>[2x]MSLNRLLSAARRSDRRASALSSFRSLSASPALAPSAASPPAPPPPTAMIYDRAAEAIKSKLRQLENPDPRFLKHGNPRPALSDHTRILAAPETRVTTLPNGLRVATESSLAARTATVGVWIDAGSRFETEETNGTAHFLEHMIFKGTERRNARELEEEIENMGGHLNAYTSREQTTYYAKVTDSDVPQALDILADILQNSRFEENRISRERDVILREMEEVEGQTEEVIFDHLHATAFQYTPLGRTILGPAQNIKTITKAHLQSYIQTHYTAPRMVIAASGAVKHEDIVEQVKKLFTKLSTDATTTAQLVAKEPAIFTGSEVRMLDDDIPLAQFAVAFEGASWKDPDSIALMVMQAMLGSWNKTAGGGKHMGSELAQRVGINEVAESIMAFNTNYKDTGLFGVYAVAKPDCLDDLSYAIMQETTKLVYRVSEDDVTRACNQLKSSLLLHIDGTSPVAEDIGRQLLTYGRRIPFAELFARIDAVDASTIKRVANRFIYDKDVAIAAMGPIQRLPDYNWFRRRTYWNRY;>[2x]MYRAAASSFRRHLKGHGSKLGSTRSSTSAAVAARTSKGGLFSWLTGERSSSLPSLDIPLGGVVLPDPLPDSVEQSKTKITTLSNGLKIASETSPNPAASIGLYLDCGSIYETPFSSGASHLLERMAFKSTTNRSHFRIVREVEAIGGNIGASASREQMGYTFDALKTYVPQMVELLVDCVRNPAFLDWEVNEELRKVKAELGELSNNPQGLLLEAIHSAGYSGALAYPLLAPEAALNRLDGPSLE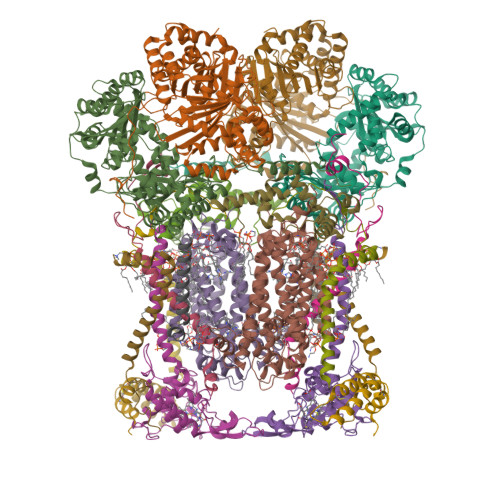EFVAENYTAPRMVLAAAGVEHEELVSIAEPLLSDLPNVPRPDEPKSVYVGGDFRRHGESGGTHVALAFEVPGGWHKEKDAIVLTVLQMLMGGGGSFSAGGPGKGMHSRLYLRVLNEYQQIQSFSAFNSIFNNTGLFGIYASTSPDFAPKAVDIAAKELIAIASPGQVTQVQLDRAKKSTKSAVLMNLESRMIASEDIGRQILTYGERKPLEQFLKAVDEITLNDITKISQKIISSPLTMASYGDVLSVPSYESVNRKFHAK;>MTIRNQRFSLLKEPISSTLNQHLIDYPTPSNLSYWWGFGSLAGICLVIQIVTGVFLAMHYTPHVDLAFNSVEHVMRDVEGGWLLRYMHANGASMFFIVVYLHIFRGLYYASYSSPREFVWCLGVVIFLLMIVTAFTGYVLPWGQMSFWGATVITSLASAIPVVGDTIVTWLWGGFSVDNATLNRFFSLHYLLPFLLVGASLLHLAALHQYGSNNPLGVHSEMDQISFYPYFYVKDLVGWVAFAIFFSIWIFYAPNVLGHPDNYIPANPMSTPPHIVPEWYFLPIYAILRSIPDKSGGVAAIALVFICLLALPFFKSMYVRSSSFRPIYQGIFWLLLADCLLLGWIGCQPVEAPFVTIGQISSFVFFLFFAITPILGRVGRGIPNSYTTDETEM[2x];>[2x]MTGGVFQLLRRKLHPQFTNSSLLSPIIAKKDGAGSTGSRSLKVLALIGAGVSGFFSFSTVAVADEAEHGLACPSYPWPHKGILSSYDHASIRRGHQVYTEVCASCHSMSLISYRDLVGVAYTEEEVKAMAAEIEVVDGPNDEGEMFTRPGKLSDRFPQPYANEAAARFANGGAYPPDLSLITKARHNGQNYVFSLLTGYRDPPAGVSIREGLHYNPYFPGGAIAMPKMLNDGAVEYEDGTPATEAQMGKDVVSFLSWAAEPEMEERKLMGFKWIFVLSLALLQAAYYRRLRWSVLKSRKLVLDVVN;>[2x]MLRVAAKRLSSLSSSAWRANHAASAVLSRNPVAPSLSTEEHRSDPFSLRPEFFLPIRGYATDSLFHPKENSLIPEIPATVAAVKNPSSKIIYDEHNHERFPPGDPSKRAFAYFVLTGGRFVYASLIRLLVLKFVLSMSASKDVLALASLEVDLSSIEPGTTVTVKWRGKPVFIRRRTEDDIKLANSVDVASLRDPQQDAERVKNPEWLIVIGVCTHLGCIPLPNAGDFGGWFCPCHGSHYDISGRIRKGPAPYNLEVPTYTFLEENKLMIG;>[2x]MASFLQSFLDPKKNWLAAQHMKSLVKRLSKYGLRYDDLYDPYYDLDVKEALNRLPKEVVDARHARLKRAIDLSMKHEYLPEDLQAMQTPFRGYLQDMLALVKRERAEREALGGLPLYQRSIP;>[2x]MGKQIVPVKSVIYALSPFQQKVMTGLWKDLPTKIHHKVSENWISATLLLGPLVGTYAYVQNYLEKEKLHHRY;>[2x]MADEEPVDQKRYLEESCKPKCVKPLLEYQACIKRIHGDDSGQKHCTGQYFDYWFCVDKCVAPKLFTKLK;>METVARRRGGGIFESLYKVVMRRNSVYVTFVIAGAFLGERAVDYGIHKLWEANNVGKRYEDIPVLGQKLSEE[2x];>[2x]MAGLPARLRIQPADVKAAAMWGVAAATGGLYLVQVSILVLPPVKVVFHFYLVSGFRICLDVKDLRTMPCSAPRIWRLYILI> GF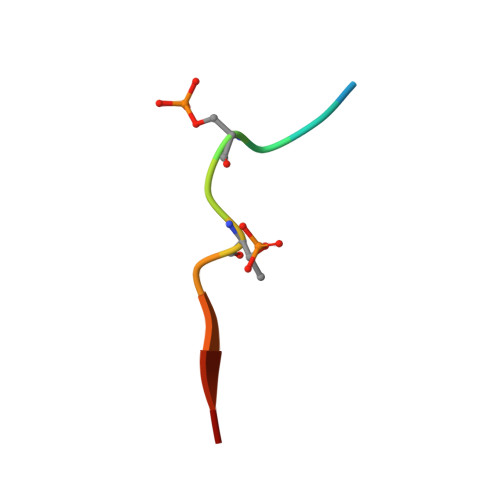IDSDTDVEEE>MAETDGSIPLIPVRMLNEHVYCPRLAYLMWVQGEFSHNEFTVDGVIRHRRVDAGGGVLPSETQEDSRIHARSVSLSSERLGITAKIDLVEGEGAYVSPVDYKRGKRPHVAGGAYEPERVQLCAQGLLLREHGFASDGGALYFVASRERVPVAFDDELIGRTLAAIDEMGRTALSGTMPPPLEDSPKCPRCSLVGICLPDEVRFLSHLSVEPRPIIPADGRGLPLYVQSPKAYVRKDGDCLVIEEERVRVAEARLGETSQVALFGNATLTTAALHECLRREIPVTWLSYGGWFMGHTVSTGHRNVETRTYQYQRSFDPETCLNLARRWIVAKIANCRTLLRRNWRGEGDEAKAPPGLLMSLQDDMRHAMRAPSLEVLLGIEGASAGRYFQHFSRMLRGGDGEGMGFDFTTRNRRPPKDPVNALLSFAYAMLTREWTVALAAVGLDPYRGFYHQPRFGRPALALDM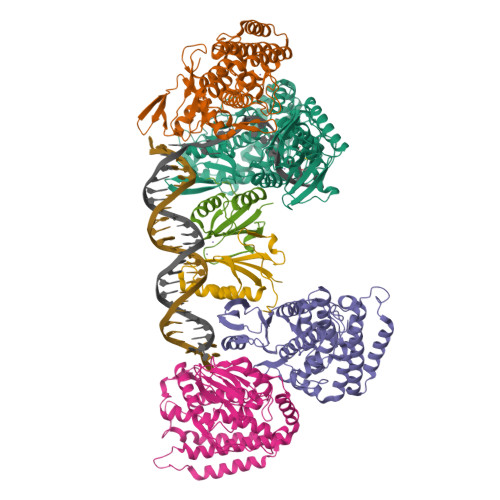MEPFRPLIADSTVLMAINNGEIRTGDFVRSAGGCNLTDSARKRFIAGFERRMEQEVTHPIFKYTISYRRLLEVQARLLTRYLSGEIPAYPNFVTR[4x];>MEHLYIVSYDIRNQRRWRRLFKTMHGFGCWLQLSVFQCRLDRIRIIKMEAAINEIVNHAEDHVLILDLGPAENVKPKVSSIGKTFDPILRQAVIV[2x]>MSTQYETQGYTINNAGRRLVVDPITRIEGHMRCEVNINDQNVITNAVSCGTMFRGLEIILQGRDPRDAWAFVERICGVCTGVHALASVYAIEDAIGIKVPDNANIIRNIMLATLWCHDHLVHFYQLAGMDWIDVLDALKADPRKTSELAQSLSSWPKSSPGYFFDVQNRLKKFVEGGQLGIFRNGYWGHPQYKLPPEANLMGFAHYLEALDFQREIVKIHAVFGGKNPHPNWIVGGMPCAINIDESGAVGAVNMERLNLVQSIITRTADFINNVMIPDALAIGQFNKPWSEIGTGLSDKCVLSYGAFPDIANDFGEKSLLMPGGAVINGDFNNVLPVDLVDPQQVQEFVDHAWYRYPNDQVGRHPFDGITDPWYNPGDVKGSDTNIQQLNEQERYSWIKAPRWRGNAMEVGPLARTLIAYHKGDAATVESVDRMMSALNLPLSGIQSTLGRILCRAHEAQWAAGKLQYFFDKLMTNLKNGNLATASTEKWEPATWPTECRGVGFTEAPRGALGHWAAIRDGKIDLYQCVVPTTWNASPRDPKGQIGAYEAALMNTKMAIPEQPLEILRTLHSFDPCLACSTH[2x];>[2x]LENKPRIPVVWIHGLECTCCTESFIRSA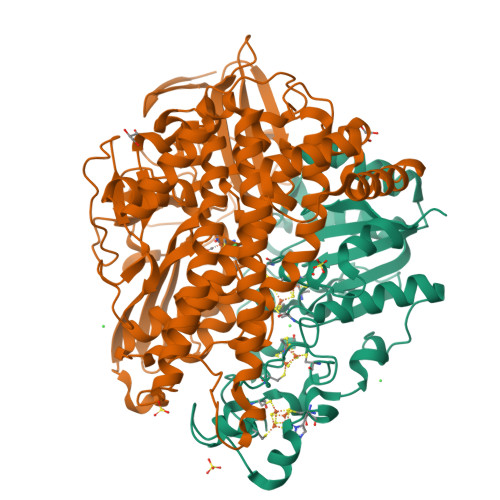HPLAKDVILSLISLDYDDTLMAAAGTQAEEVFEDIITQYNGKYILAVEGNPPLGEQGMFCISSGRPFIEKLKRAAAGASAIIAWGTCASWGCVQAARPNPTQATPIDKVITDKPIIKVPGCPPIPDVMSAIITYMVTFDRLPDVDRMGRPLMFYGQRIHDKCYRRAHFDAGEFVQSWDDDAARKGYCLYKMGCKGPTTYNACSSTRWNDGVSFPIQSGHGCLGCAENGFWDRGSFYSRVVDIPQMGTHSTADTVGLTALGVVAAAVGVHAVASAVDQRRRHNQQPTETEHQPGNEDKQARSHHHHHH>GSCPHTYKPVCGANGEVYDNECFLNKAGIEPAESWETCRG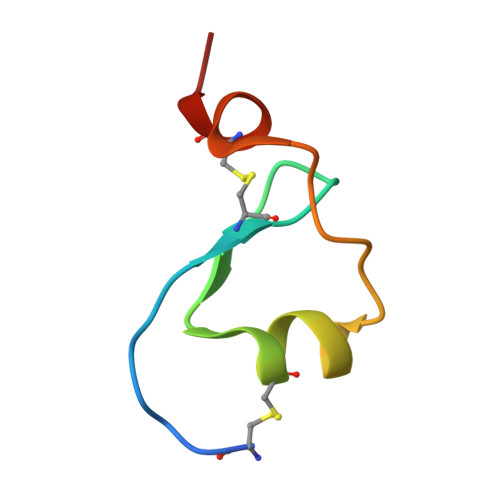HE[2x]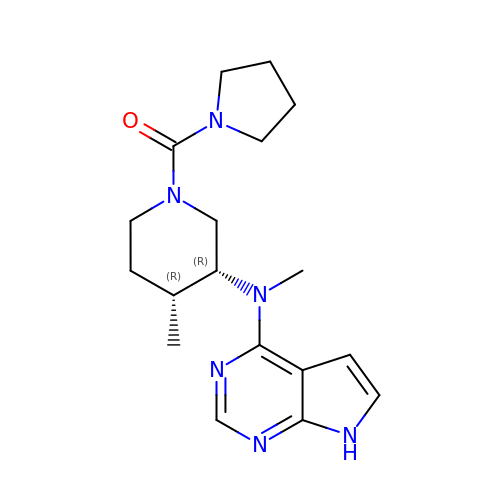{(3R,4R)-4-methyl-3-[methyl(7H-pyrrolo[2,3-d]pyrimidin-4-yl)amino]piperidin-1-yl}(pyrrolidin-1-yl)methanone | C18 H26 N6 O | RONMOMUOZGIDET-HIFRSBDPSA-N> MTHLPGNIYTLFTPVNGPKSKDEWIDTSKIMLDLHIDNMSSSDYIPSAIDRTDLVMVQSVHLLRKTGGRGLFAREDIPKGTCIGIYTGEVYSEQEFEQYLKEHVGSDKSYAMYVGGRVIDAARKGNLTRYINFSDSQDNAEFVETTLNRKKVAKVITTKNIKAGQQLLINYNTYEEQASRYYYFLNPGDGWLSAQ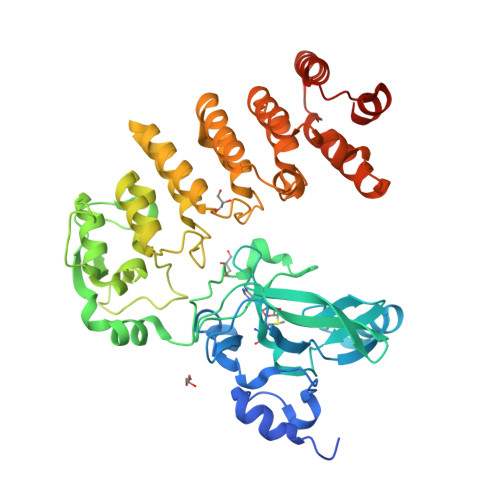EFYQTYQSQYRLEQMPYNLEGFDLKAGDRVLMTQIGRIILANYSLAKEQELNASDIDLPFLKVGSDEKILDFDEADTFTPLMAACYLGQVENVKWLIEHGANIDQQQSHSGHCPLSLTLKGYSLAKDTQKYIDIIQLLIKNQVNLLVHDRSDKTFLHNAALVLNNLDFQSVVKFLIGQNPIDINEYFTYIDENDFDIVMHCYNNKLFDKALVLLAFYPDYFKRNYMSDNEGHNQFNINAFRKAIKDFNSNERSILLMQLRESGLHLPEDLLEQLGIMDSSITLESKFF> GPDEIDLSALRDPAGIFELVELVGNGTYGQVYKGRHVKTGQLAAIKVMDVTGDEEEEIKQEINMLKKYSHHRNIATYYGAFIKKNPPGMDDQLWLVMEFCGAGSVTDLIKNTKGNTLKEEWIAYICREILRGLSHLHQHKVIHRDIKGQNVLLTENAEVKLVDFGVSAQLDRTVGRRNTFIGTPYWMAPEVIACDENPDATYDFKSD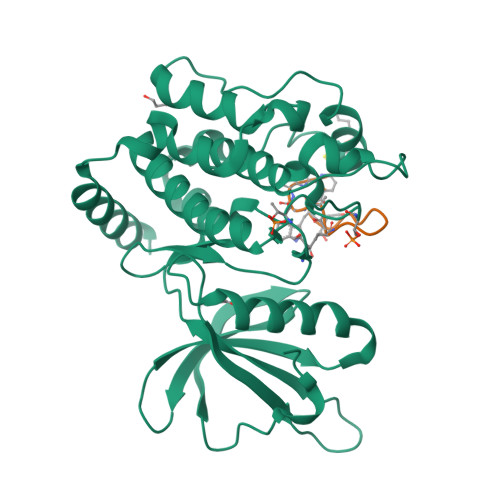LWSLGITAIEMAEGAPPLCDMHPMRALFLIPRNPAPRLKSKKWSKKFQSFIESCLVKNHSQRPATEQLMKHPFIRDQPNERQVRIQLKDHIDRTKKKRG;> SWGFIYKTLKSSGSCSCX[5-(bromomethyl)-1-benzothiophen-2-yl]-tris(oxidanyl)boranuide 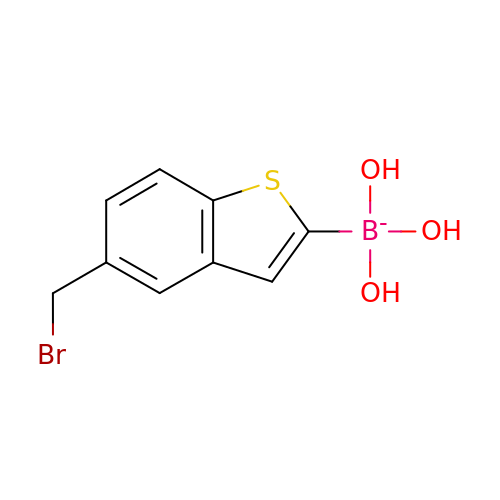| C9 H9 B Br O3 S | YBCAXTUNRJBXIK-UHFFFAOYSA-N> MTLGPVVTGTSVIAIKYKHGIMIAADRKASYGSYAKFQNVERIFKINNKTVMGFSGELADAQYLHELLTRKNINNLSEKKRKEDMYTPQHYHSYVSRVFYVRKNRIDPLFNNIIIAGINSQKYDNNDDNVLLYTNKNNDDEQNEYKNNEEYKEIHKDDLYIGFVDMHGTNFCDDYITTGYA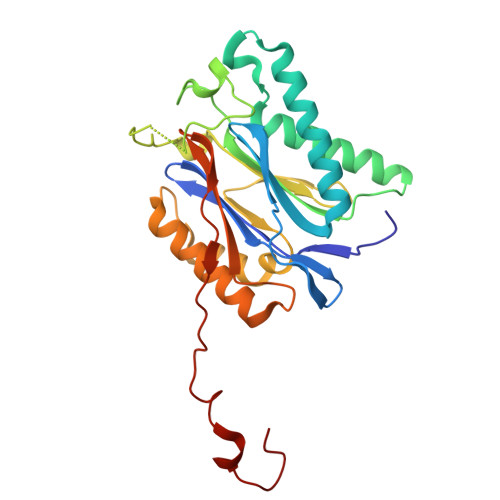RYFALTLLRDHYKDNMTEEEARILINECLRILYFRDATSSNFIQIVKVTSKGVEYEEPYILPCVLNSADYVYPSTLLPPAGCMW> SMGIINQVSTVTKVIHHELEVAASADDIWTVYSWPGLAKHLPDLLPGAF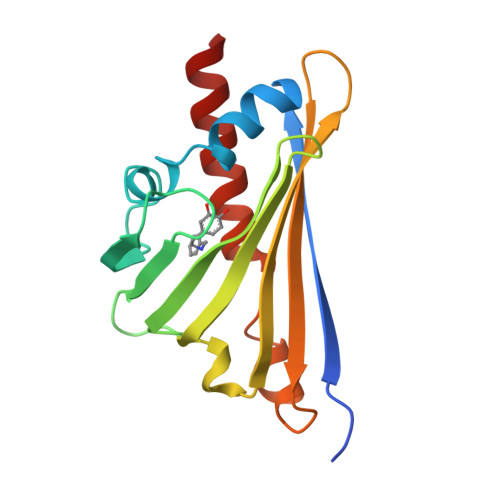EKLEIIGDGGVGTILDVTFVPGEFPHEYKEKFILVDNEHRLKKVQMIEGGYLDLGVTYYMDTIHVVPTGKDSCVIKSSTEYHVKPEFVKIVEPLITTGPLAAMADAISKLVLEHKS>[2x]GSSPSLEQDDGDEETSVVIVGKISFCPKDVLGHGAEGTIVYRGMFDNRDVAVKRILPECFSFADREVQLLRESDEHPNVIRYFCTEKDRQFQYIAIELCAATLQEYVEQKDFAHLGLEPITLLQQTTSGLAHLHSLNIVHRDLKPHNILISMPNAHGKIKAMISDFGLCKKLAVGRHSFSRRSGVPGTEGWIAPEMLSEDCKENPTYTVDIFSAGCVFYYVISEGSHPFGKSLQRQANILLGACSLDCL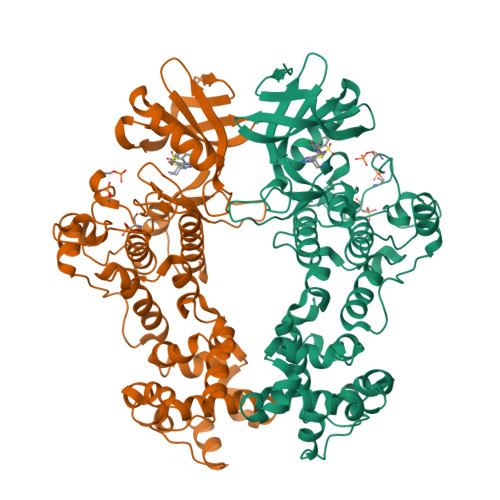HPEKHEDVIARELIEKMIAMDPQKRPSAKHVLKHPFFWSLEKQLQFFQDVSDRIEKESLDGPIVKQLERGGRAVVKMDWRENITVPLQTDLRKFRTYKGGSVRDLLRAMRNKKHHYRELPAEVRETLGSLPDDFVCYFTSRFPHLLAHTYRAMELCSHERLFQPYYFHEPPEPQPPVTPDALGNS> MHHHHHHSSGLEVLFQGPGSVPLPAGWEMAKTSSGQRYFLNHNDQTTTWQDPRKAMLSQLNVPAPASPAVPQTLMNSASGPLPDGWEQAMTQDGEVYYINHKNKTTSWLDPRDRPPPYVAPPSYEGPHRTLG

WW domains organize molecular assemblies by binding to short, proline rich peptide motifs each with ~4–6 residues. The type I WW domains bind to a consensus ‘PPxY’ motif (where P is proline, x is any amino acid and Y is tyrosine, also known as PY-motif) with very modest affinities (with Kd in the range of a few to a few tens of µM). To achieve this goal, we determined the high resolustion structures of 7 representative WW tandem/target complexes, and measured the binding constants of >100 WW domain tandems or isolated WW domains binding to known or previously unknown targets. In this study, we discovered that WW tandems, but not individual WW domains, can bind to target proteins with extremely high affinity and with very high sequence specificity.

The two WW domains of YAP are also arranged next to each other forming a WW domain tandem. We were able to obtain high diffraction quality crystals when the Dendrin PY23 sequence was fused to either the N- or C-termini of the YAP WW tandem. We solved the structures of these two versions of the complex. Although each WW domain engages the ‘PPxY’ motif following the canonical type I WW/target bindings, the overall structure of the YAP WW tandem/Dendrin PY23 complex differs substantially from those of the KIBRA/MAGI2 WW tandems in complex with the same ligand (Figure 3E vs Figure 3F for example) in two distinct aspects. First, the inter-domain linker of the YAP WW tandem is unstructured and there is no C-terminal helix following YAP WW2. Thus, the two WW domains of YAP do not form a supramodule due to very limited inter-domain contact. This is supported by the two versions of the complex structures solved, in which the inter-domain orientations are obviously different. Second, the Dendrin PY23 binds to the YAP WW tandem in a parallel orientation (i.e. PY2 binds to WW1 and PY3 binds to WW2), instead of the antiparallel binding orientation observed for the KIBRA/MAGI2 WW tandems. This is again likely attributed by the lack of inter-domain interactions between the two WW domains of YAP so that each domain can freely choose its more preferred PY-motif.> MHHHHHHSSGRENLYFQGSTLSYTLGQLAAHVGAEVRGDADLPIQGLATLQEAGPAQLSFLANPQYRKYLPESRAGAVLLTAADADGFAGTALVVANPYLAYASLSHLFDRKPKAAAGIHPTAIVAADAEVDPSASVGAYAVIESGARIGAGVSIGAHCVIGARSVIGEGGWLAPRVTLYHDVTIGARVSIQSGAVIGGEGFGFANEKGVWQKIAQIGGVTIGDDVEIG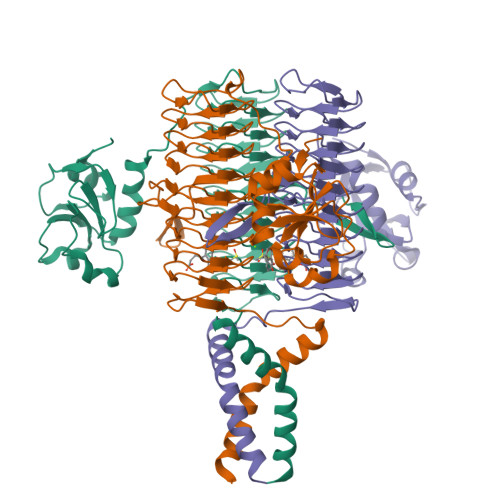ANTTIDRGALSDTLIGNGVKLDNQIMIAHNVQIGDHTAMAACVGISGSAKIGRHCMLAGGVGLVGHIEICDNVFVTGMTMVTRSITEPGSYSSGTAMQPAAEWKKSAARIRQLDDMARRLQQLEKRLAAVTSSGDASSD(1R)-4-acetamido-3-amino-1,5-anhydro-2,3,4-trideoxy-1-sulfo-D-glycero-D-galacto-octitol 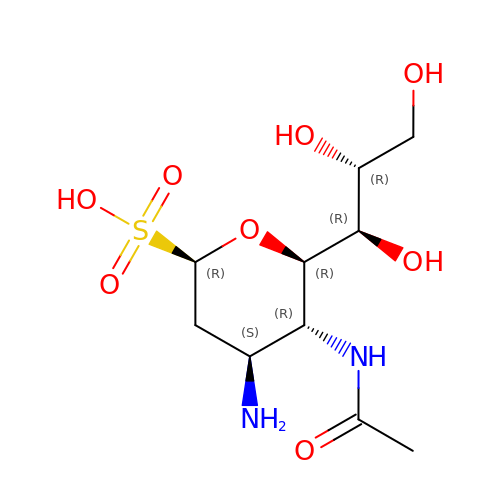| C10 H20 N2 O8 S | XAZGDFCTWHWJMA-IHICSVBISA-N>[3x]MAGIVTEPWSVAEN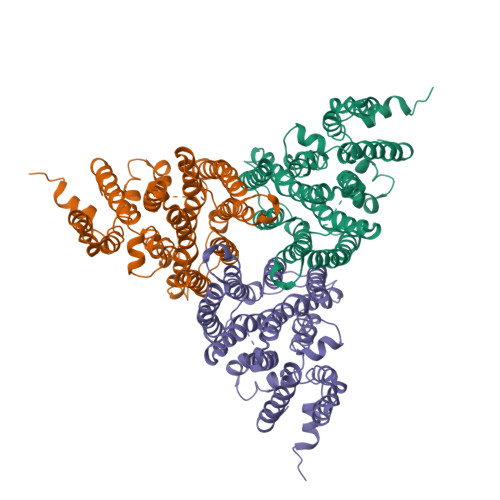GNPSITAKGSSRELRLGRTAHNMDDDDLRKKSDLRVIQKVPYKGLKDFLSNLQEVILGTKLAILFPAIPAAIICTYCGVSQPWIFGLSLLGLTPLAERVSFLTEQLAFYTGPTLGGLLNATCGNATELIIAILALTNNKVAVVKYSLLGSILSNLLLVLGTSLFCGGIANIRREQRFDRKQADVNFFLLLLGFLCHLLPLLVGYLKNGEASAAVLSDMQLSISRGFSIVMLISYIAYLVFQLWTHRQLFDAQEQEDEYDDDVEQETAVISFWSGFAWLVGMTLVIALLSEYVVATIEEASDKWNLSVSFISIILLPIVGNAAEHAGAVIFAFKNKLDISLGVALGSATQIGLFVVPLTIIVAWILGINMDLNFGPLETGCLAVSIIITAFTLQDGSSHYMKGLVLLLCYFIIAICFFVDKLPQKQNAIHLGHQAMNNVVTATGGGVFSSDYKDDDDK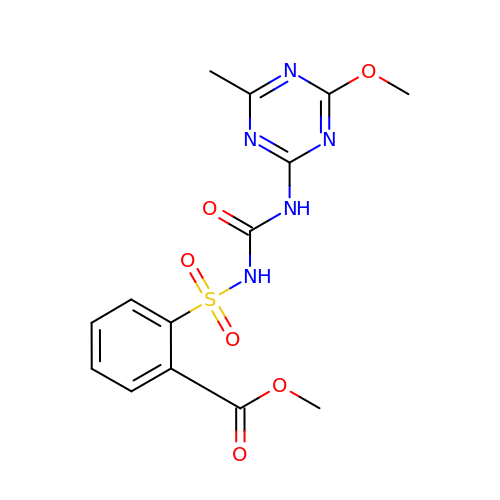METHYL 2-[({[(4-METHOXY-6-METHYL-1,3,5-TRIAZIN-2-YL)AMINO]CARBONYL}AMINO)SULFONYL]BENZOATE | C14 H15 N5 O6 S | RSMUVYRMZCOLBH-UHFFFAOYSA-N Here we show that a rhoptry-resident kinase RON13 is a key virulence factor that plays a crucial role in host cell entry. Cryo-EM, kinase assays, phosphoproteomics and cellular analyses reveal that RON13 is a secretory pathway kinase of atypical structure that phosphorylates rhoptry proteins including the components of the RON complex. RON13 is a 153 kDa type II transmembrane protein with a putative serine/threonine kinase domain and a large luminal carboxy-terminal extension (CTE) with no identifiable structural motif. Ultimately, RON13 kinase activity controls host cell invasion by anchoring the moving junction at the parasite-host cell interface.

The canonical HRD catalytic triad of ePKs differs in RON13 with an HFD motif conserved among all the coccidian orthologues of RON13. In addition, ATP hydrolysis activity was detected. The catalytic activity was completely abolished by introducing a single amino acid change (D595A) in the catalytic HFD motif (rRON13dk), validating the importance of this conserved kinase motif for enzymatic activity. To gain insight into the function and regulation of RON13 kinase, its three-dimensional structure was resolved at 3.1 Å resolution by single-particle cryo-EM. The RON13 kinase domain is similar to ePKs, but contains an α-helical N-lobe insertion (NLI) present exclusively in RON13 coccidian orthologues. Unlike ROPKs that also reside in the rhoptries, RON13 lacks an α-helical N-terminal extension. The kinase C-lobe structure contains all the motifs required for ATP transfer to the substrate, as well as a ROPK-specific disulfide bond. The CTE is mainly composed of α-helices clamping the kinase domain C-lobe. Of note, the CTE is essential for RON13 folding and stability as neither expression of the kinase domain alone, nor proteolytic cleavage to separate the kinase domain from the CTE of rRON13 yielded a functional RON13 kinase. Cleaved rRON13 behaved exactly as WT rRON13 when analyzed by size-exclusion chromatography, further emphasizing the strong interaction between RON13 kinase domain and the CTE. Analysis of RON13 electrostatic potential highlighted a rather extended positively charged groove lying on one side of the kinase that may be involved in protein–protein interactions, but did not provide strong hints to the role the CTE plays. Of interest, three autophosphorylation sites were identified on RON13: Thr379 and Ser381 within the NLI in proximity to the ATP-binding site (N-lobe) and Thr703 closer to the activation loop (C-lobe).

> GAGTTGGKKDDQALSFLGDTKSASELNPPRLVCPDKPPTLPPREEQVRKAYALPLCELPWDDLGPMLGSGTFGRVYPLRRPACTEVTKGFVGRKFAVKIFWLKRKGMMNLFDTISQGGTPSAEQTDPGTIAAIKSEIRSLPTSSSAFRDMVRIADPTVDVEKIKGMADSLTVETIMKEAKTLRTVINTNGFYTEVGETGTIFTQMEKFVQAHRPEIWSTLSKASQEAQASKYAEIGLADNHWSLPLARVLVKDKNDVKHWALLIELFDGDLQPKTDKTGYSLDGWNAKSGGNVVLREIFSSREALIGLTSKLVKPFVVMQNLYSLGHFAIKPPNLLYKYFPGEKGRASRLSVAAGDFGMAGLLHGDMILRGTLAFMAPEMERVSGGLVAKPSYDVYALALTLASFWTAATELRDHYPWVEKCIKPTLKKMKDAPEFTFLRFASKTGPKLYEADTIYALSTCFAVGGKVEKLYHTGMPLLIRLKLSQMADPEPLARVSMRHARFVFKAYAMLDKLLRAPQSEANAETREEQLKQLQSLHIVQFLLFYLRMEPLTAARDNTQSYRRLARALLDFARLDPVYQAATETVQPLPYEFFTEQKDWQNVKVEVSGSEVDETIRKLRTSLTRDRSLSEDSWADLVDIMFGVSLDGLREVVTRVVYSRKTFLLEEKIGNAVKEAVAATYKFDPNTQLIAEDAPDRLFEVVRTDLGLSYPDDSELGRFLVHRVSKSHTAWATVDRLARQALRLALRREERTRQVYEQLLSGEKPSSESEKAFFDSVFSAVSVVSEANYFGLFWDFPSAGLFGVPPEEMQAYVRKTHLAFVGKMWPVETQKKILEAAVRVTVRGLNASLPASLVDVYATVFAALPTKAPVSPPFLYGLEREEYSSLLFDAKLPEFKEMVAFWATRHELNIAVQTAVGKIPDATNLSDEDIEKQLEGMLPAHLRSPSPARFGWPPEAVADNIRLFIREAKDELALHGPDMVHNRIRVNGRSKPPRRAAFLFHEIFRKAIAFKKDISVLQFNQFFTDILKQSFDPQCRRFIAEVKKRVKSAPAEYVRVADTEAVAPLFEGEGKDILKLVAVDPAARASDPEPNNCFLWTQAFLDDKTIVVSTGSSGSSGHHHHHHHHHH> GGLEKDFLPLAFGWFLTKKSSETLRKAGQVFLEELGNHKAFKKELRHFISGDEPKEKLELVSYFGKRPPGVLHCTTKFCDYGKAAGAEEYAQQEVVKRSYGKAFKLSISALFVTPKTAGAQV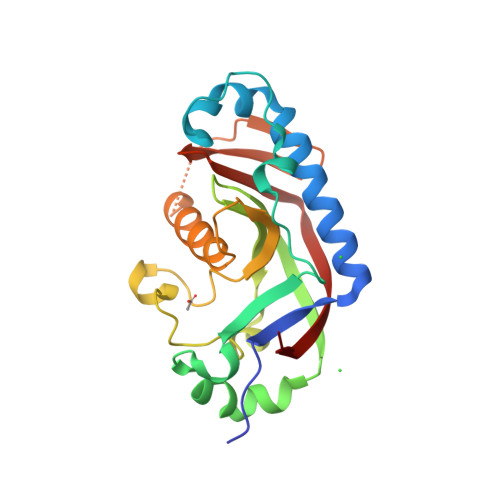VLTDQELQLWPSDLDKPSASEGLPPGSRAHVTLGCAADVQPVQTGLDLLDILQQVKGGSQGEAVGELPRGKLYSLGKGRWMLSLTKKMEVKAIFTGYYG Light-oxygen-voltage (LOV) proteins form a sensory photoreceptor class that elicit a wide palette of physiological responses to blue light across archaea, bacteria, protists, fungi, and plants. Likely via a radical-pair mechanism, T1 reacts within microseconds to the signaling state, characterized by a covalent thioadduct between a highly conserved cysteine residue in the LOV photosensor and the C4a atom of the flavin isoalloxazine ring system. Thioadduct formation entails a hybridization change of the flavin C4a atom from sp2 to sp3 and concomitant protonation of the adjacent N5 atom. A highly conserved glutamine residue in strand Iβ is situated immediately adjacent to the flavin and has been identified as instrumental in reading out the flavin N5 position and eliciting the downstream transitions.

To arrive at a molecular understanding, we solved the crystal structures of AsLOV2 wild-type and Q513L in the dark-adapted states to resolutions of 1.00 Å and 0.90 Å, respectively. In dark-adapted AsLOV2 Q513L, the flavin plane was displaced by ~0.4 Å relative to the wild-type protein, arguably due to steric interactions between the flavin O4 and the Cδ2 methyl group of L513. Notably, no ordered water molecules entered the space vacated by the glutamine removal. The resultant loss of hydrogen bonds at the flavin O4 atom may account for the hypsochromic absorbance shift evidenced above across the different LOV receptors with replaced glutamine. The Q513L replacement notwithstanding, the crucial N414 residue assumed the conformation seen in darkness for the wild type, i.e., engaged in hydrogen bonds with D515 and the backbone carbonyl O of residue 513. Interestingly, the Q513L dark state showed alternate conformations for the Aβ-Bβ and Gβ-Hβ loops, in the case of the wild-type receptor only seen upon light exposure. We note that neither the dark-adapted nor the light-adapted structures of AsLOV2 Q513L revealed direct evidence for ordered water molecules near the flavin N5 atom.

> GEFLATTLERIEKNFVITDPRLPDNPIIFASDSFLQLTEYSREEILGRNCRFLQGPETDRATVRKIRDAIDNQTEVTVQLINYTKSGKKFWNLFHLQPMRDQKGDVQYFIGVLLDGTEHVRDAAEREGVMLIKKTAENIDEAAKEL The penicillin-binding proteins (PBPs) synthesize and remodel the cell wall peptidoglycan, a major component of the bacterial cell wall that gives the cell its shape and rigidity. In E. coli, PBP3 (FtsI) is an essential protein of the divisome, catalyzing peptide cross-bridges between the glycan chains of the peptidoglycan. The overall fold of periplasmic PBP3 is bimodular. The C-terminal module is responsible for the transpeptidase activity but no clear function has been assigned yet to the N-terminal module of the construct.

The crystal structure of a soluble form of PBP3, including residues 57 to 577, was solved at 2.5 Å resolution. PBP3 crystallizes in space group P6122 with one molecule in the asymmetric unit. The structure was built from residues 71 to 567 but absence of detectable electronic density did not allow structure determination for residues 93–112, 119–141, 152–162, 202–228 and 537–543. The active site responsible for the transpeptidase activity of PBP3 is located in a long groove that can accommodate the carboxy-terminal residues of the PBP3 natural substrate, the peptidoglycan stem pentapeptide L-Ala-γ-D-Glu-meso-diaminopimelic acid (mDAP)-D-Ala-D-Ala. The transpeptidase activity of PBP3 relies on eight residues, Ser307, Lys310, Ser359, Asn361, Lys494, Thr495, Gly496 and Thr497, found with few exceptions in all penicillin-binding enzymes. In PBP3, the oxyanion hole, defined by the amine groups of residues 307 and 497, is unexpectedly occupied by the hydroxyl group of Tyr514 that is at 2.7 Å from Ser307N and 3.25 Å from Thr497N. The side chain of Tyr514 is free to easily rotate and liberate the oxyanion hole and should not play a particular role in transpeptidation. Electron density around residues 499–510, a loop that connects strands β3 and β4 close to the active site, is weak but sufficient to allow its determination. The N-terminal module provides three loops (180–190; 202–228; 280–294) and one subdomain (88–165) for potentially interacting with other proteins of the divisome. Because domain swapping in the PBP357–577 crystal would involve a large twisting of the (88–165) domain and, also, because domain swapping should stabilize the domain and hence provide a clear electronic density in that region, the domain swapping observed in the case of PBP388–165 is probably absent in the PBP357–577 crystal.

> VSTSRGMITDRSGRPLAVSVPVKAIWADPKEVHDAGGISVGDRWKALANALNIPLDQLSARINANPKGRFIYLARQVNPDMADYIKKLKLPGIHLREESRRYYPSGEVTAHLIGFTNVDSQGIEGVEKSFDKWLTGQPGERIVRKDRYGRVIEDISSTDSQAAHNLALSIDERLQALVYRELNNAVAFNKAESGSAVLVDVNTGEVLAMANSPSYNPNNLSGTPKEAMRNRTITDVFEPGSTVKPMVVMTALQRGVVRENSVLNTIPYRINGHEIKDVARYSELTLTGVLQKSSNVGVSKLALAMPSSALVDTYSRFGLGKATNLGLVGERSGLYPQKQRWSDIERATFSFGYGLMVTPLQLARVYATIGSYGIYRPLSITKVDPPVPGERVFPESIVRTVVHMMESVALPGGGGVKAAIKGYRIAIKTGTAKKVGPDGRYINKYIAYTAGVAPASQPRFALVVVINDPQAGKYYGGAVSAPVFGAIMGGVLRTMNIEPDALTTGDKNEFV>ALVPRGSIKKCLFPAAGYGTRFLPATKAMPKEMLPVVNKPLIQYAVEEALEAGLSEIGIVTGRGKRSLEDHFDISYELEHQIRNTDKEKYLVGIRRLIDECTFAYTRQVEMKGLGHAILTGRPLIGDEPFAVVLADDLCLNLEGDSVLKQMVKLYNQFRCSIVAIQEVPPEETNKYGVIAGEMIRDDIFRVNTMVEKPKPEEAPSNLAIIGRYILTPDIFDLIEQTEPGKGGEIQITDALMKQAQDGCVLAYKFKGKRFDCGSAEGYIEATNFCYENLYKTGKAH[8x]

The enzyme uridine diphosphate (UDP)-glucose pyrophosphorylase (UGP, EC 2.7.7.9) occupies a key position in UDP-sugar metabolism as it converts glucose-1-phosphate (Glc-1-P) and uridine triphosphate (UTP) to inorganic pyrophosphate (PPi) and UDP-glucose (UDP-Glc); the latter, in turn, can be converted into UDP-glucuronic acid, UDP-galactose, and UDP-galacturonic acid. In the search for new treatment options, P. aeruginosa uridine diphosphate-glucose pyrophosphorylase (PaUGP) has been proposed as a novel drug target because it is required for the biosynthesis of important virulence factors and linked to pathogenicity in animal models. To establish a basis for the development of selective PaUGP inhibitors, we solved the product-bound crystal structure of tetrameric PaUGP and conducted a comprehensive structure-function analysis, identifying key residues at two different molecular interfaces that are essential for tetramer integrity and catalytic activity and demonstrating that tetramerization is pivotal for PaUGP function. Importantly, we show that part of the PaUGP oligomerization interface is uniquely conserved across bacterial UGPs but does not exist in the human enzyme, therefore representing an allosteric site that may be targeted to selectively inhibit bacterial UGPs.

The crystals have the symmetry of monoclinic space group P1211 and diffracted to 2.9 Å resolution. The crystal structure comprises residues 1–279 of PaUGP, of which we were able to successfully model residues 1–275; the C-terminal residues were not modeled due to weak electron density. Each PaUGP subunit contains one UDP-Glc molecule and one Mg2+ ion in the active site. The crystals of PaUGP contain eight molecules per asymmetric unit; however, through analysis of crystal contacts, it was possible to reassemble the biologically active homotetramer as seen in HpUGP. Each PaUGP subunit contains an open twisted central β-sheet surrounded by α-helices on both sides with a total of 12 α-helices and 12 β-strands, resembling the Rossman-fold characteristic for nucleotide-binding enzymes. Using symmetry-related objects, we reconstructed the biologically active PaUGP homotetramer as seen in HpUGP, which can be described as a dimer of dimers, with subunits A/B as well as C/D forming “tight” dimers, and A/C as well as B/D forming “loose” dimers, respectively. Subunits A and B, as an example of the tight dimer, are packed with a burial of 2,005 Å2 of solvent-accessible surface. As in HpUGP, subunits A and C, as an example of the loose dimer, are less densely packed with a total buried accessible surface of 1,054 Å2; however, a tight hydrogen bond (H-bond) network is established between four charged amino acids.> MHHHHHHHHHHSGQNLYFQGHMATFISVQLKKTSEVDLAKPLVKFIQQTYPSGGEEQAQYCRAAEELSKLRRAAVGRPLDKHEGALETLLRYYDQICSIEPKFPFSENQICLTFTWKDAFDKGSLFGGSVKLALASLGYEKSCVLFNCAALASQIAAEQ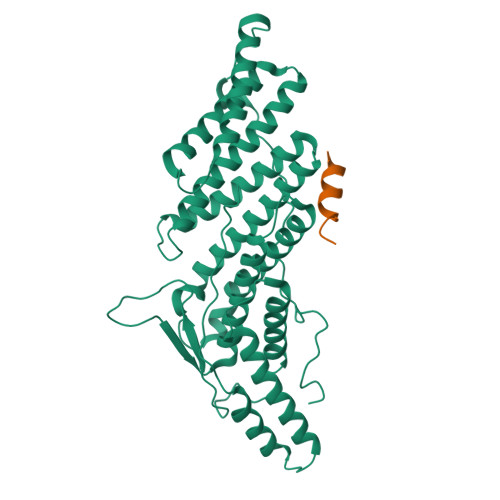NLDNDEGLKIAAKHYQFASGAFLHIKETVLSALSREPTVDISPDTVGTLSLIMLAQAQEVFFLKATRDKMKDAIIAKLANQAADYFGDAFKQCQYKDTLPKEVFPVLAAKHCIMQANAEYHQSILAKQQKKFGEEIARLQHAAELIKTVASRYDEYVNVKDFSDKINRALAAAKKDNDFIYHDRVPDLKDLDPIGKATLVKSTPVNVPISQKFTDLFEKM;> QRAEEEDDDIKQLAAWTT>[12x]SMGRRCQAQVSRRISFSASHRLYSKFLSDEENLKLFGKCNNPNGHGHNYKVVVTVHGEIDPATGMVMNLADLK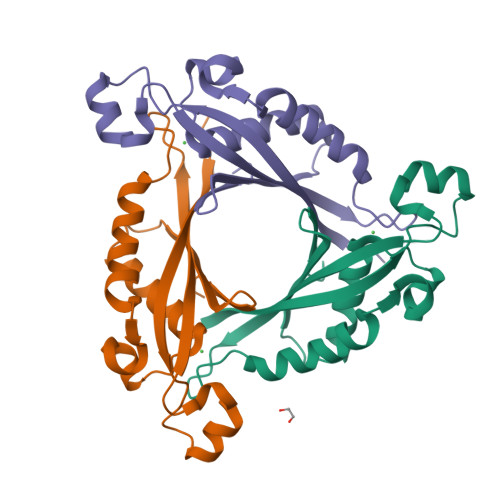KYMEEAIMQPLDHKNLDMDVPYFADVVSTTENVAVYIWDNLQKVLPVGVLYKVKVYETDNNIVVYKGE>[4x]MKLKTNIRHLHGIIRVPGDKSISHRSIIFGSLAEGETKVYDILRGEDVLSTMQVFRDLGVEIEDKDGVITVQGVGMAGLKAPQNALNMGNSGTSIRLISGVLAGADFEVEMFGDDSLSKRPMDRVTLPLKKMGVSISGQTERDLPPLRLKGTKNLRPIHYELPIASAQVKSALMFAALQAKGESV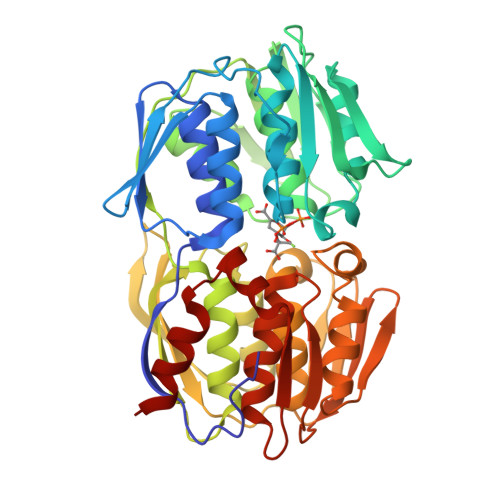IIEKEYTRNHTEDMLQQFGGHLSVDGKKITVQGPQKLTGQKVVVPGDISSAAFWLVAGLIAPNSRLVLQNVGINETRTGIIDVIRAMGGKLEITEIDPVAKSATLIVESSDLKGTEICGALIPRLIDELPIIALLATQAQGVTVIKDAEELKVKETDRIQVVADALNSMGADITPTADGMIIKGKSALHGARVNTFGDHRIGMMTAIAALLVADGEVELDRAEAINTSYPSFFDDLESLIHG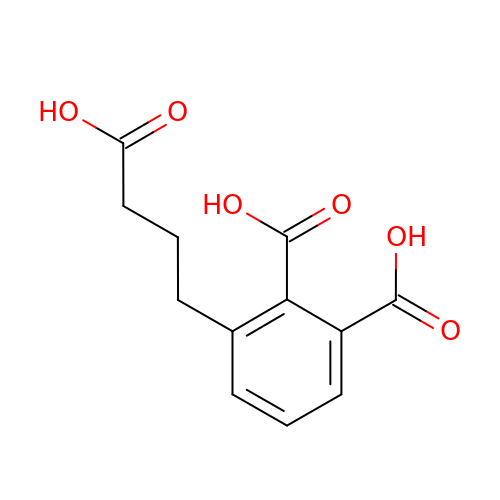3-(3-carboxypropyl)benzene-1,2-dicarboxylic acid | C12 H12 O6 | IPHJRPHIMBNGTQ-UHFFFAOYSA-N Viral transcription is highly regulated, as demonstrated biochemically in viruses of the Reoviridae. mRNA transcription in these viruses is activated by external actions, for example, removal of their outer shell in multi-shelled reoviruses and binding of S-adenosyl-L-methionine (SAM) in the single-shelled cytoplasmic polyhedrosis virus (CPV). To reveal the mechanisms of transcriptional regulation of viruses within the Reoviridae family, we determined the cryoEM structures of six CPV/ligand complexes in the presence of magnesium ion: CPV+SAM (i.e., ‘S-CPV’), CPV+SAM+4 nucleoside triphosphates (NTPs) (i.e., transcribing, or ‘t-CPV’), CPV+SAM+GTP+ATP (i.e., ‘SGA-CPV’), CPV+SAM +GTP (i.e., ‘SG-CPV’), CPV+GTP (i.e., ‘G-CPV’), and CPV+ATP (i.e., ‘A-CPV’) at resolutions ranging from 2.9 to 3.1 Å. Like the atomic model of unliganded CPV, the atomic models of these liganded CPV all contain two conformers of the capsid shell proteins (CSP-A and CSP-B), two conformers of the large protrusion proteins (LPP-3 and LPP-5), and one conformer of TP in each asymmetrical unit. We discovered that the large sub-domain of guanylyltransferase (GTase) domain of CPV turret protein (TP) also has an ATP-binding site and is likely an ATPase that mediates the activation process of viral RNA transcription and capping.

First, through incubating CPV capsids with SAM, GTP, ATP, and Mg2+, we obtained the SGA-CPV particle which, lacking of UTP and CTP, is incapable of mRNA transcription. Indeed, under cryoEM, SGA-CPV, and S-CPV particles look similar and differ from actively transcribing t-CPV particles. However, the 3.1 Å structure of SGA-CPV shows global movements and local conformational changes of its structure proteins that are indistinguishable from those of t-CPV. Furthermore, the large sub-domain of SGA-CPV GTase domain also contains a ligand similar to that in the t-CPV. In t-CPV and SGA-CPV, two SAM molecules bind to the MT-1 and MT-2 domains, one Mg2+-GTP to the GTase site and one ATP to the putative ATPase site. Second, the GTase domains in SGA-CPV and SG-CPV are also in the open state with prominent densities attributable to Mg2+. Located on the same side of the leaving group (i.e., β, γ-diphosphate), His208 is hydrogen bonded to the β-phosphate of the GTP in SGA-CPV and SG-CPV. (C) The distance between Nε2 of His217 and the α-phosphorus of GTP in SGA-CPV is ∼4.5 Å. The distance between the Nε of Lys234 and the α-phosphorus is ∼7.8 Å.

> MWHYTSINNDTRVALDPKPNQIRTITKPNTVPQLGTDYLYTFNSQRRSHTLRLLGPFQYFNFSETDRGHPLFRLPLKYPSKAIPADELIDNLHSWMRSVHLLHVRSEDNTLRYNWMLGVYARSTNYTTPVGQLVVNAPAILNYSNPQDAFNSVFVALGIDYIDIPITNSNIFDDSSTPYNVRIWHAPTMTEVNHILALMRKSTLVSTHSSWHWNVLHTFHYRSESDMIDHFAAKILEDWRQKEKLDKGALVEADRVIQRLIPLSSSTYVQRLAAIGALYPNEFTENVLDLSRLSTALLQLSDTYYQHANDQLRRLYRRMYNDSRTLYMTQRHQELLLAQITADPNILLYPYTYIFTTIPTSMNYISNTGQGRIKHSLTVTGATEHDTVADIVLGQTGEDVITISMVEPMSIAVEDMYGYVLDTPTRDIWPADEQIEQKGDAVALYDTKTSRALGMFNNTVRIDDLLSPLLSLVYRTYIKGDTMTMTQGSLDHLTLCAAVDSDITFVGNRMIAPLPEGYIPKPMHRNNSTMKMLSLYVALKKLENFATNSYLMAPDTSIILLGAEREPAVNILRRFNRNVSNVRIIGMGDRAVEPNIRVRVPFPIDKNISADFIICDINSYEDQSFESMFSETISVVTTCASAATRALVKINHPSEYMINSVIERLSQLGGVFYHTALLKTASQNPYSYETYIYITPIAAAVRFPFYSNSAMINRYMTAVADDEMPIIPSIHTVIKGHSNTYSPGLFCGCVDVQSAPLALSQLKSYCSEATTWRVDSDDNLVNIIARIDPARIALEFRTRSNTSAYHEYQRYVPNGLGFKVRKTREFRYMHREVTFIHKLMMYALIREQISLTENMTQVVSIGGRNLADISVVPLNMKYVVIDPATRIETLTQEKKNIEVQSRPFQFDAANMDLENNSIYLFIAVIMNEPNGAATPARMQMDKIRNVATAMLTRTNCVAYISFYEAGIITRLDQSTAHKTIRVEEGRLKVANYVPVDTLVEADVTLMLRDIGITHEIIRPSTPELIDACSNYGIRLGSTGGAVLDVFNHYSPVIKLVRS;>[2x]MHSTNNNSNKRNNEEKHKQPEIDSSANNGEGTSGTRAQTVGDTATEAGVRNETEAGASTRRQTDGTGLSGTNAKIATASSARQADVEKPADVTFTIENVDDVGIMQQKKPPTVVQSRTDVFNEQFANEALHPTTKVIFNGLDVNTEVQPLSDDFKQISDPKGYLTYSVKYEDQFTKKDKLRASEADDRIVGPTVNLFKYGAAVVNIDLNRDFFDTATGIDLTKGIPLVQDLLVPIGVTAGAEQSAEYVSGLLMVLFKVMTDNRLVIVGETTTPMSNTLSTVVNNVLRTTYHNNVGVNPALLRDFTQVNWLNRDITNMLQQAGTKYGLGLTETRLDYVRLVKTIVGHALNIDHFAASVLNINLRALMEANVTADDRIKALQAHSMISTQFHGPNQGALRPELAFDHDHIIRCLMLAAANYPRLEGIIVQINTGYVASANVIRPVSEKRYFPENLEQNQSAARLVSAVKARASEADISSIHLAIAREVSPMFNVHELKKIAESFEDPSSIVVVLEFILFALFFPTEFNRIKGDIQNVLLLFFSRWYPVEYGIFVQRGATYTINAAGEFEFSGRNEKWDQALYLSEHFPALFSDVPLAGANTIIAIMRLFTPQGFLRTDDLAIAANFPRASRNPQTYIPYTNQRGTVTNEFASRFRTIVATLANVVNERAVQDDMQKATRSCTKQWLRHLETQFDNIAVAHTDHLSVVYATMSNFMLNFTNNFSGNHATFKPDQYVITSPEGSYKPIIERQGETVDGLTIIDTSIVWPILCQCTYPLVRQSGKGVDAVSIMEEIVYPDPSTTLSQSLSVAQVLSKLTLPDAFINMILSGGDSVVMRTYQTEADDDLDEGIRMTTYDQYLSHIRERLHITNVPDPIYITGASTPDQIAASVQATHVAVVLYQSGVINGPASTYLRENEVLVVMPDYYDVVSRFANANLQMNNNRYHESVLEIADIFDQADFIQTSDAVRQLRALMPTLSTSQIRHAIERIAQITDVDSTDYGKLTLRFLGTLTRSLKMQNAQIRRIRPDGTVLRYDDQIDIEAFRWSRYFLDELQLRRLSVGLRLITNPRIARRFNGVRIMYLTDDDPDPDFVPDVPEGYVAVQYAHRLFSSSLANKRNRVTYTHPPTGMAYPSPTGRPHVHMTINERAGMSKLVADNIIASVIKSNWVVDILDIEYTAEVMTPSEGYTQHVDAESIMTAPKGKLFHLQFMDGLLRPEPSAFDPPASGEDMRLIYPLQPISVARSMRAIVNHNEVDRPRGAVAPSSYEMDTGTLSRNGDLLYSPVANGQVGIPKLEVDHISFSNVVSMMTANIRTGDDMAVERVNPDDVRAINIRNA;>[2x]MLQQPTGGYTTLEQFAFTIRNDGTNATPTQFLQLLSYEATENELVKKTIPTPETHLPSARNVPGNVYIEDAITQALFGISAQNVNAHGYFSRLSALALPNTSARLGLDGVIYNSETINIPFYDPAAVANFAATYAKLGNASTPRYRADMIDIYAHVGLELAGTDAERAAGVMPVKRAKFDSWEGSLISLSRDVVNWKILAFLIDLCSLEGEALRAFKTRNRDVFRMMLFIMSTAVAANVVNRKVTKRVDRVLEYIGVNSMRTAGRTATITYDLSRHEFAAKFLQLTFTRWNAASAMIRSMPDMHTPRTSITPAGENALVRHNRYMTENFKGLSPIALAQKKHEMMLHTHEIHSMDIDGSIKNMVERETVNKMNEIDAMNTAPWTEEFAEVEPTTVYERHQIGTDPEQTQLISQDAAVIVHQASSDVDENEYGNSVSELTIDTQSDSVL> SHSTAETTLDSFFSRAGLVGEIDLPLEGTTNPNGYANWDIDITGYAQMRRKVELFTYMRFDAEFTFVACTPTGQVVPQLLQYMFVPPGAPEPDSRESLAWQTATNPSVFVKLSDPPAQVSVPFMSPASAYQWFYDGYPT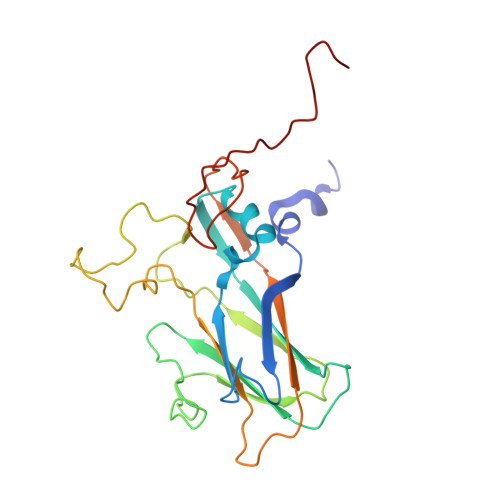FGEHKQEKDLEYGACPNNMMGTFSVRTVGTSKSKYPLVIRIYMRMKHVRAWIPRPMRNQNYLFKANPNYAGNFIKPTGASRTAITT>[4x]MAPLETIYDESLNKSADSIDDKKWSKLFPRIVSDPDRSSNFMTRAIYVAFSAVLRNRNILGQEYFTKNYITEKLKCMTLCFRNLRSNQIAQLLRNAGDATKDGFLKEVSLVITNNEGDLEAIEVFSMKFIYFENGGVVARLSTDKNGQEDPHFAKLAQLVYEGGDSV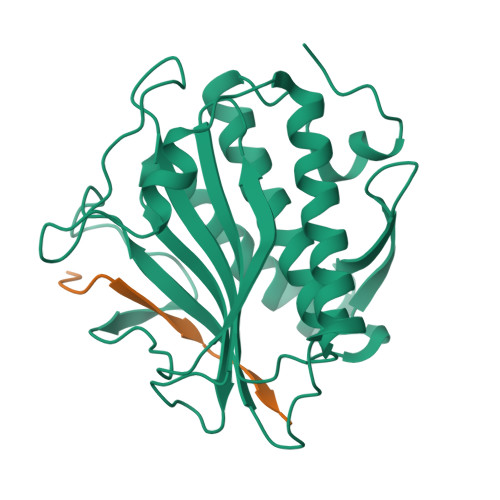RDQMVTIVRSVQFLCTKVLEPLPEEFTANFRLEYTNDAPSNFRIDGFEDSSTFYTLPDDIQSATIGHLRPGCHAANMECWSMLMSD;>[4x]SNARDSPYGLSQGITKKNKD> RGSHHHHHHGSVKIVTSQAEFDSIISQNELVIVDFFAEWCGPSKRIAPF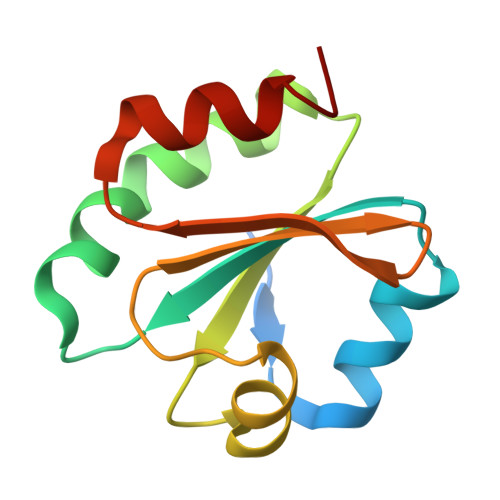YEECSKTYTKMVFIKVDVDEVSEVTEKENITSMPTFKVYKNGSSVDTLLGANDSALKQLIEKYAA Annexin A2 is a non-EF-hand calcium-binding protein that is characterized by the ability to bind and aggregate (i.e. ‘annex’) anionic phospholipid membranes. AnxA2 preferentially binds to phospholipids and other anionic polymers and does not contain any canonical RNA- or DNA-binding motifs. Importantly, AnxA2 was shown to bind phosphorothioate oligonucleotides and has been implicated in the release of PS ASOs from endo-lysosomal compartments in productive ASO cellular trafficking. In the present study, we co-crystallized the C-terminal domain (CTD) core of AnxA2 with a PS 2′-MOE DNA gapmer ASO and found that unique hydrophobic interactions between PS groups and lysine and arginine residues account for the enhanced affinity of PS ASO to the protein surface.

From our crystallization trials, we obtained two types of AnxA2–ASO co-crystals that were used to solve two structures referred to as structure I and structure II, determined at 1.9 and 2.4 Å resolution, respectively. The asymmetric unit of structure I contains one AnxA2 protomer and two chains of ASO. For one DNA strand, all 15 nucleotides were clearly visible, whereas for the second strand, 10 nucleotides could be built in the model. Unexpectedly, partial complementarity of the ASO region that encompasses nucleotides 2–10 promoted intermolecular base pairing. As a result, two strands form a largely ordered duplex in the structure. The key interaction is formed between loop IIIAB (the convex surface of AnxA2) and the phosphorothioate between nucleotides dT14 and dG15 close to the 3′ end of the DNA. This part of the ASO adopts a distorted conformation that allows the phosphorothioate linkage to interact with a pocket on the surface of the protein that is created by R205 and K206. The interaction is primarily mediated by contacts between the backbone and aliphatic parts of both amino acid side chains that make van der Waals contacts with the PS group. Closer inspection of the binding site clearly demonstrates that the interactions with lysine and arginine residues in this structure would only be possible when the non-bridging sulfur is in the Rp position of the PS stereoisomer. Distinct electron density from the calculated difference map was clearly visible around the phosphorus atom and Rp non-bridging atom in the inspected PS linkage, which unambiguously confirmed that only this PS stereoisomer is bound at this site.

> SDAERDALNIETAIKTKGVDEVTIVNILTNRSNAQRQDIAFAYQRRTKKELASALKSALSGHLETVILGLLKTPAQYDASELKASMKGLGTDEDSLIEIICSRTNQELQEINRVYKEMYKTDLEKDIISDTSGDFRKLMVALAKGRRAEDGSVIDYELIDQDARDLYDAGVKRKGTDVPKWISIMTERSVPHLQKVFDRYKSYSPYDMLESIRKEVKGDLENAFLNLVQCIQNKPLYFADRLYDSMKGKGTRDKVLIRIMASRSEVDMLKIRSEFKRKYGKSLYYYIQQDTKGDYQKALLYLCGGDD>[7x]MTDSVQTETTEGKIIINLFAPNLPGSTKEDDLIQKSLRDQLVESIRNSIAYPDTDKFAGLTRFIDESGRNVFFVDGTRGAGKTTFINSVVKSLNSDQDDVKVNIKCLPTIDPTKLPRHEPILVTVTARLNKMVSDKLKGYWASNDYRKQKEQWQNHLAQLQRGLHLLTDKEYKPEYFSDALKLDAQLDYSIGGQDLSEIFEELVKRACEILDCKAILITFDDIDTQFDAGWDVLESIRKFFNSRKLVVVATGDLRLYSQLIRGKQYENYSKTLLEQEKESVRLAERGYMVEHLEQQYLLKLFPVQKRIQLKTMLQLVGEKGKAGKEEIKVKTEPGMQDIDAIDVRQAIGDAVREGLNLREGSDADMYVNELLKQPVRLLMQVLQDFYTKKYHATSVKLDGKQSRNERPNELSVPNLLRNALYGSMLSSIYRAGLNYEQHRFGMDSLCKDIFTYVKQDRDFNTGFYLRPQSESEALRNCSIYLASQVSENCQGSLSKFLQMLLVGCGSVSIFNQFVTELARAENDREKFEQLISEYVAYMSVGRIESASHWANRCCAVVANSPNDEKIGVFLGMVQLNRKSRQHMPGGYKKFNIDTENGLAKAAMASSLSTVASNNLMDFCSVFNLIGAIADISACRCERSAITNAFNKVIAQTTCIVPPWSEAAVRAEMKGSSKSADNDAAVLDVDLDPKDDGVIDESQQDDATEFSDAITKVEQWLKNVNEIEIGIRPSALLIGKVWSRFYFNLN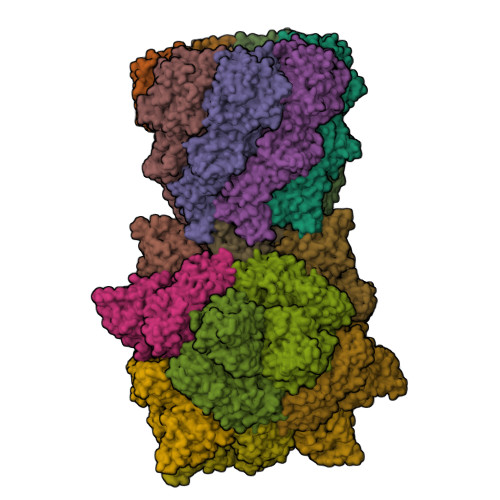NVADQHKTRLYRNAEHGRMASQSNAAKIMRFNVLAFLHAVLVEESLYHSVSDREYIGEGLRLNPVTSVDEFEKKIKIIGEKLKADNKTWKNTHPLFFLLISCPILHPFIFPVGGINCSVKALNKETSFNKLIDEIVGDKLLSDEEWDYLTKNNDQKTNTRQQIFQNTITSLNSSTIVGASYDKDTPARKTKSPLLGDSEEK;>MERFLLNSTVLLYRLSTVSLDEVSLDERVESSVFLAQYEQARSLPDHVAKSAWSYLVQQIKQRNMKLGPVAILRLIAEKFIKNEKGGPKIDLPMFSEWQTLMSRVSCLPIIACHQVFNPGPASQEYSFRWPLYPYHPTVEDYITRECLHETHQHLNGSTSAEECWLDALKHPEACLRDFEKGWASQEMKQLCAQIDPSLTPRIFKDRLQIACNIREILCRVAQGVELPEWIASMQNPQQLANSTILHNGREYGFATVWPIDDKYSQESEFCWLTGLLEKWRFNAPEGLERLLWIYLLIQNQYLTLLVQRDDFFGFEQFQNYTMTELREETEKSYLSRFKHAHGAGVYSQVRYLEGRFAPKSDPNKMQKLLFSVLRGYWEYLSAHMSMEWVHEKPLTISQVLDNLELVEPHGKCVELALVPHFIKRKPKNGEAYPHALLFKDLKNQAAILMDMLKSEPRLTGWIRGVDAAANEMHAPPELFCPLFRVLAKSGIAHFTYHVGEDFPHLISGIRSIDDALRFLPLRNGDRLGHCTAIGITPSIWKRSLPLSLSMTKETRLLDLVFIWRELRSHPELLRYASDAAIEAVRLAHKVFSLEEEVSITTLDQVFEMRGLLAESEGLLSELNEPLKPKSLWLEEYERARELVKTTGMKRPLKLYKQWLTSDNVRKQRAEYVEVALEYLPDEAVVALQQAVMAKMADRNIAIECPPTSNTRISQYRNVSEHHIFRWMGLPGEAIEGDVPMSICLGSDDPGIFAADLKSEFYHLFVVLTRKFGLSPADALRKVAEVNENGRIYRFHDVS[12x]> GAMVMRLGDAAELCYNLTSSYLQIAAESDSIIAQTQRAINTTKSILINETFPKWSPLNGEISFSYNGGKDCQVLLLLYLSCLWEYYIVKLSQSQFDGKFHRFPLTKLPTVFIDHDDTFKTLENFIEETSLRYSLSLYESDRDKCETMAEAFETFLQVFPETKAIVIGIRHTDPFGEHLKPIQKTAANWPDFYRLQPLLHWNLANIWSFLLYSNEPICELYRYGFTSLGNVEETLPNPHLRKDKNSTPLKLNF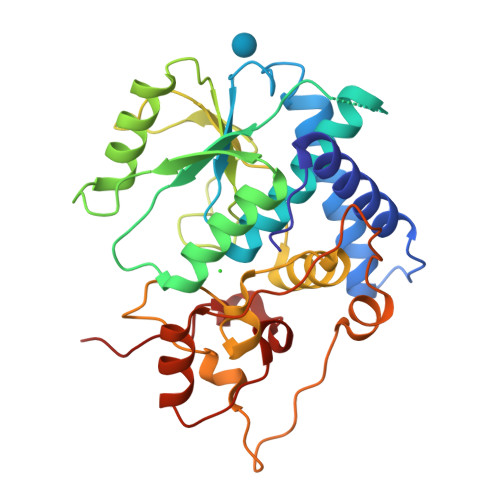EWEIENRYKHNEVTKAEPIPIADEDLVKIENLHEDYYPGWYLVDDKLERAGRIKKK> SLGLAQSAQEILDRVEKNLSTPWQATVQGRIQGPGGEEELLARVYALPQARLFRVEFLKPGSLEGNFTVITEKEVWNYLYLTNQLVISPREKAKIQGLGFAP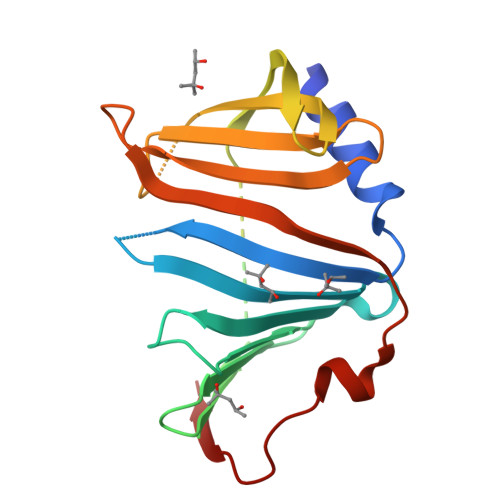QGLGDLKALSEQVDLRLEGEVRLPEGMAWKLVGRSKENQGFAAMELYILKADPRPLRFVFLDEKGKVLADLKVVEFKRTNLTEAQLKRYPKDAQVVRR>[2x]MSYNNPNNSNSHLRPHAYNNSRRDDSDGDESSIEFLNQRSNTPLTQGTYNYHNTSTNSLNFQQPEPIYRNQTRTSLSDSYYDHPIFDTSQTQIQPPHDNPFTESYEMTDTSYQGNDHHYRTGQPNHLMNPTYNQAFIPHVYDEEDNDEQEYDQRIQYNQFQGDHFDLAAISYADDESQSQLDYVPTERVIPEGEEEEEEGETSFEKEPGSETISGPFGEERSFEEPPPQQEVRSKKLTRATGLNGHLVLDCPVADELLSKFPDYNPAEKSGGLSREFAFMRYTAVTCGPSNFYRDAYILRPVHYPIPRQTELMIVITMYNEDDILL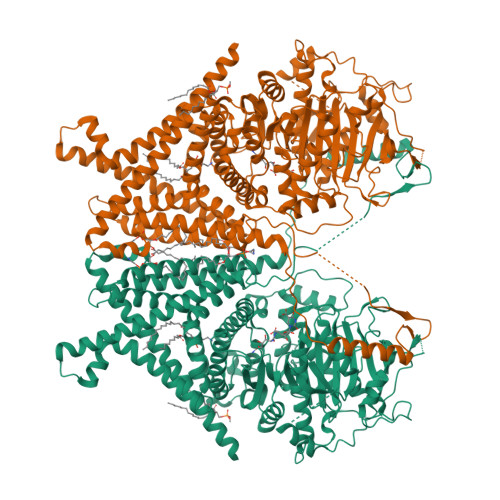GRTLKGVFKNIKYLESKARSSTWGKDSWKKIVVCIVSDGRTKINERAQALLAGLGVYQEGLAKSRVDDKKVQAHMFEYTTRVGISKVTDDVVKLTTEKVVPVQMLFCLKETNAKKINSHRWCFQAIGQVLDPKIVVLLDCGTQPSGRSLYELWKEFDRDHRVAGACGEITTSLKKRQMITNPLVYGQNFEYKISNILDKPTESSFGFISVLPGAFSAYRFIALQNDINGVGPLEKYFKGEFLHSSGELDPNDDEFQMKHLMLKEEAGIFTSNMYLAEDRILCFELVAKRGCNWLLRYCKSARAETDVPEGLAEFILQRRRWLNGSFFAAIYSLVHFYKVWTSSHSFGRKIFLHIEFFYQLINLIVSWFSIGSYFLVFRILTTSLGDKALGFAPGKILSVIFLWLYLASIVTTFVLSFGNKPKGTEKFYVTIVIFFAILMAYMIFAAIFMAVHSIQDIYRSGTRITVSLFFQNSEFRDLVVATSSTYALYFLASFLYFEPWHMFTSFVQYILLSPSYVNVLNIYAFCNIDDISWGTKGEVGGKSLGEAKLREDGTFDVSVPISKEQINQSYLDQLEKIRDPAPPEEKVLVTNTEDYYAFIRSMTVLVWMFTNFVVIALVLETGGFNQFVEATDLANLKSNRAAVFLTVILWTVAFMALFRFIGCIYYLITRLGREIKASEHATKANSLEVLFQGPDYKDDDDKAHHHHHHHHHH> MLSPPRRKAFKKWTPPRSPFNLVQETLFHDPWKLLIATIFLNRTSGKMAIPVLWKFLEKYPSAEVARTADWRDVSELLKPLGLYDLRAKTIVKFSDEYLTKQWKYPIELHGIGKYGNDSYRIFC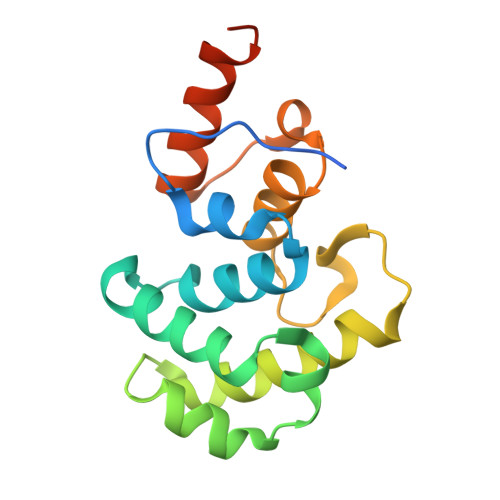VNEWKQVHPEDHKLNKYHDWLWENHEKLSLSHHHHHH>[2x]MATEPKAGRPSDYMPEVADDICSLLSSGESLLKVC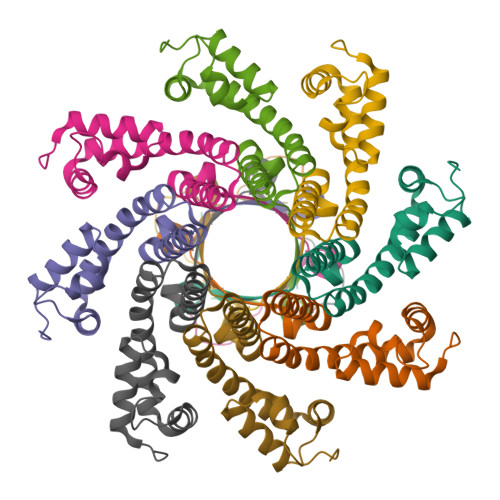KRPGMPDKSTVFAWLAKHEDFRDKYAKATEARADSIFEEIFEIADNAIPDAAEVAKARLRVDTRKWALARMNPRKYGDKVTNELVGKDGGAIQIETSPMSTLFGK>ACGLVASNLNLKPGECLRVRGEVAPDAKSFVLNLGKDSNNLCLHFNPRFNAHGDA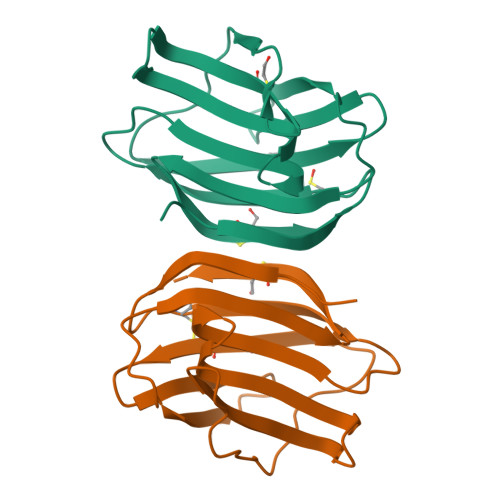NTIVCNSKDGGAWGTEQREAVFPFQPGSVAEVCITFDQANLTVKLPDGYEFKFPNHLNLEAINYMAADGDFKIKCVAFD[2x]> APADRLKALVDAAVQPVMKANDIPGLAVAISLKGEPHYFSYGLASKEDGRRVTPETLFEIGSVSKTFTATLAGYALTQDKMRLDDRASQHWPALQGSRFDGISLLDLATYTAGGLPLQFPDSVQKDQAQIRDYYRQWQPTYAPGSQRLYSNPSIGLFGYLAARSLGQPFERLMEQQVFPALGLEQTHLDVPEAALAQY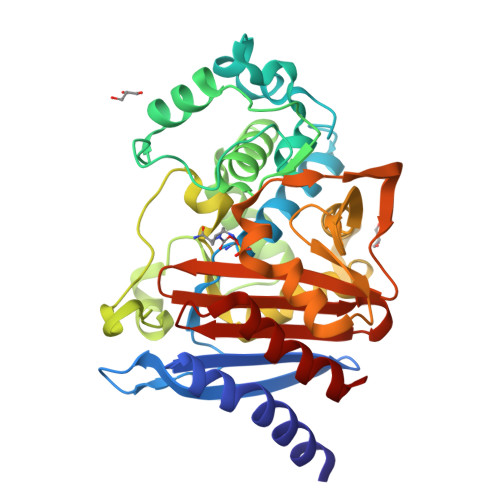AQGYGKRDRPLRVGPGPLDAEGYGVKTSAADLLRFVDANLHPERLDRPWAQALDATHRGYYKVGDMTQGLGWEAYDWPISLKRLQAGNSTPMALQPHRIARLPAPQALEGQRLLNKTGSTNGFGAYVAFVPGRDLGLVILANRNYPNAERVKIAYAILSGLE3-[3-[[4-(pyridin-2-yloxymethyl)phenyl]methyl]-1,2-oxazol-5-yl]pyridin-2-amine | C21 H18 N4 O2 | 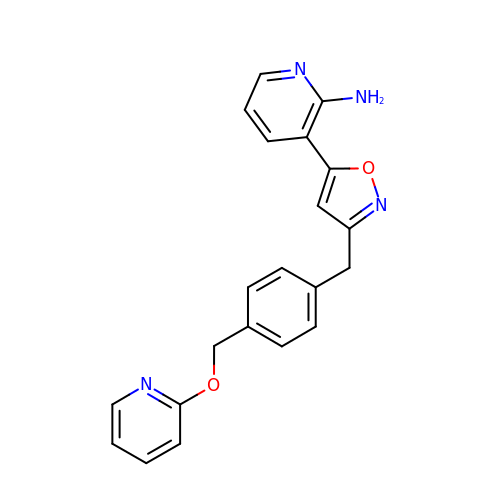WSEKTEUGRLFBSE-UHFFFAOYSA-N>STNLVAEPFAKLEQDFGGSIGVYAMD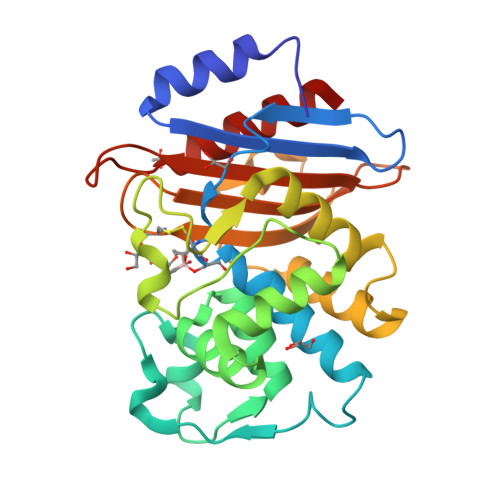TGSGATVSYRAEERFPLCSSFKGFLAAAVLARSQQQAGLLDTPIRYGKNALVPWSPISEKYLTTGMTVAELSAAAVQYSDNAAANLLLKELGGPAGLTAFMRSIGDTTFRLDRWELELNSAIPGDARDTSSPRAVTESLQKLTLGSALAAPQRQQFVDWLKGNTTGNHRIRAAVPADWAVGDKTGTCGVYGTANDYAVVWPTGRAPIVLAVYTRAPNKDDKHSEAVIAAAARLALEGLG[4x]>[8x]MPQDPSTRSSPARLLIPEPRAGRARHAACVLLAVCFVVLFLSGEPLAPITRRVCTQLAALQLGVLLKGCCCLAEEIFHLHSRHHGSLWQVLCSCFPPRWHLALLLVGGSAYLDPPEDNGHSPRLALTLSCLCQLLVLALGLQKLSAVEVSELTESSKKNVAHGLAWSYYIGYLKVVLPRLKECMEEISRTNPMLRAHRDTWKLHILVPLGCDIWDDLEKADSNIQYLADLPE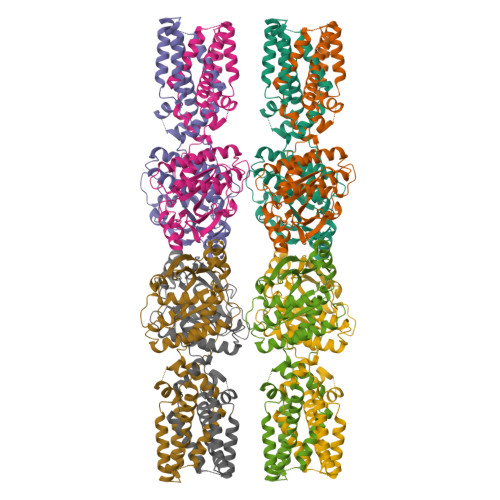TILTRAGIKRRVYKHSLYVIRDKDNKLRPCVLEFASPLQTLCAMSQDDCAAFSREQRLEQARLFYRSLRDILGSSKECAGLYRLIAYEEPAEPESHFLSGLILWHLQQQQREEYMVLEVLFQGPVDFDKTLTHPNGLVVERPVGFDARRSAEGFRFDEGGKLRNPRQLEVQRQDAPPPPDLASRRLGDGEARYKVEEDDGGSAGSEYRLWAAKPAGARWIVVSASEQSEDGEPTFALAWALLERARLQSSHHHHHHHH>[6x]TKPVHLWTKPDVADWLES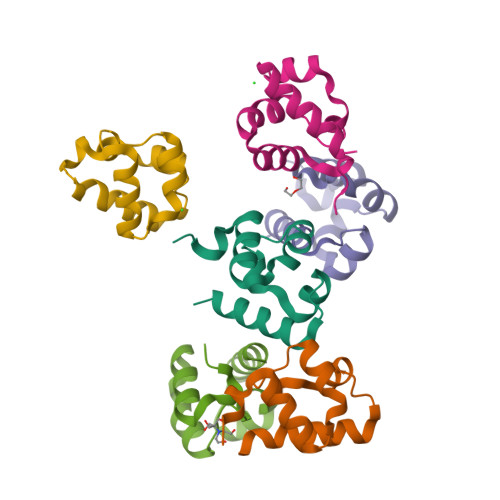LNWGEHKEAFMDNEIDGSHLPNLQKEDLIDLGVTRVGHRMNIERALKQLLDR>[2x]GSHMVKLSSKNLDARLDTVYD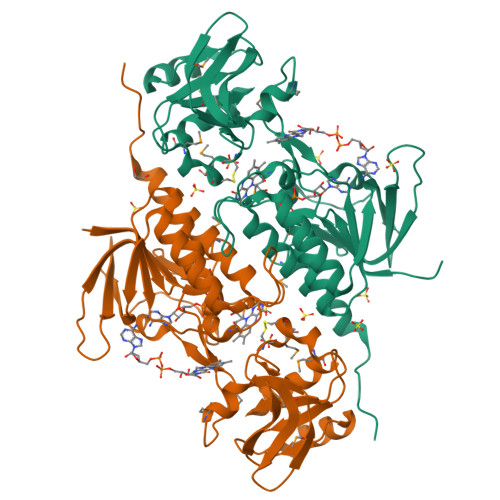AIVLGGGMGGLSAAIYLARYGLKCLVVEKGRGRSFWMQDLRNYVGLDPDTPGRDIITHSTQQALHWGADLLRGYVEDVTDEGDTLAVKVKVGKKDSLYPIFRTKYVIAATGIIDNLPQLEDMQNVYDYAGYTLHVCMICDGFDMWDQKAVLIAGTEGQINAAFVLNWFTPYITVLTHGLCTVGDEMKAKLADHGYPLHEAAITKFLGEDHKMSGVELVDGTVMEATTGLINMGSVYHNHYLKGIEGLEWDGENLVTNDMAQTSHPRIFALGDLKKGLNQVSVAVADGTLAATQIWRNIRRASEPRKWIH> MNGWNFQELKETPSQTGGPYVHIGLLPKQANIEVFEHNLDNNLVQDNTQGQRIRLEGQV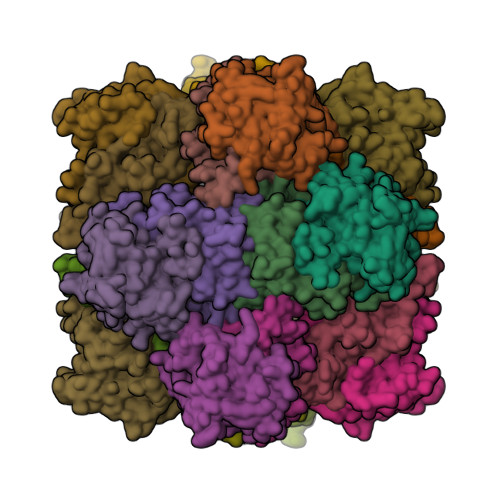FDGLGLPLRDVLIEIWQADTNGVYPSQADTQGKQVDPNFLGWGRTGADFGTGFWSFNTIKPGAVPGRKGSTQAPHISLIIFAHGINIGLHTRVYFDDEAEANAKDPVLNSIEWATRRQTLVAKREERDGEVVYRFDIRIQGENETVFFDI;> MSQIIWGAYAQRNTEDHPPAYAPGYKTSVLRSPKNALISIAETLSEVTAPHFSADKFGPKDNDLILNYAKDGLPIGERVIVHGYVRDQFGRPVKNALVEVWQANASGRYRHPNDQYIGAMDPNFGGCGRMLTDDNGYYVFRTIKPGPYPWRNRINEWRPAHIHFSLIADGWAQRLISQFYFEGDTLIDSCPILKTIPSEQQRRALIALEDKSNFIEADSRCYRFDITLRGRRATYFENDLT>MSAPHLDDRVLASLQEVMEDEYPVLLDTFVLDSEERLRSLHAALQAGDAQALRHTAHSFKGGSSNMGAVLLAGYCKELEE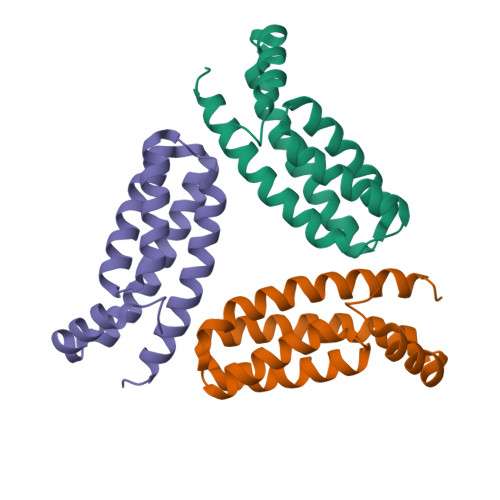SARRGELQRAPALIEQMEREFAIVRILFKQERQRYR[6x]> YQQDQVVKEDNIEAVGKKLHEYNTQFQEKSREYDRLYEDYTRTSQEIQMKRTAIEAFNETIKIFEEQCQTQERYSKEYIEKFKREGNETEIQRIMHNYEKLKSRISEIVDSRRRLEEDLKKQAAEYREIDKRMNSIKPDLIQLRKTRDQYLMWLTQKGVRQ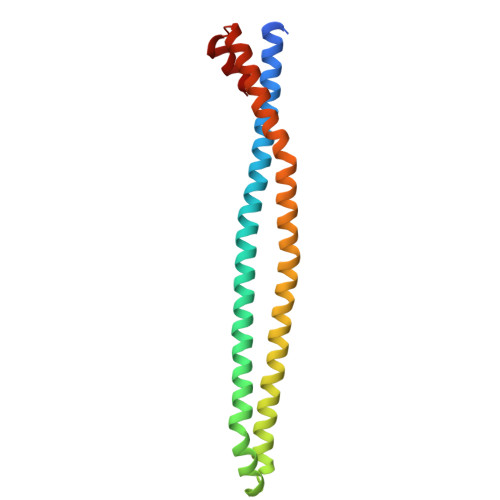KKLNEWLG>[4x]LSSSPSEILQELGKGSTHPQPGVSPPAAPAAPGPKDGPGETDAFGNSEGKELVASGENKIKQGLLPSLEDLLFYTIAEGQEKIPVHKFITALKSTGLRTSDPRLKECMDMLRLTLQTTSDGVMLDKDLFKKCVQSNIVLLTQAFRRKFVIPDFMSFTSHIDELYESAKKQSGGKVADYIPQLAKFSPD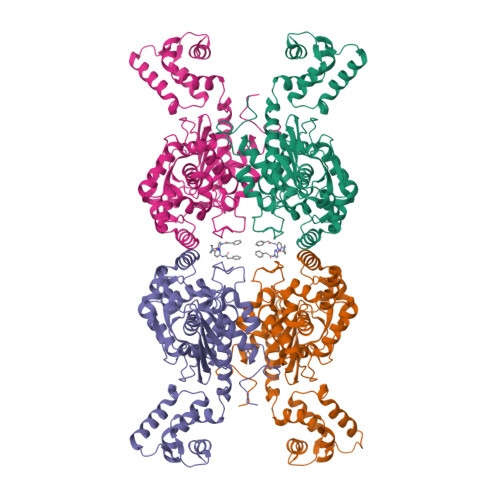LWGVSVCTADGQRHSTGDTKVPFCLQSCVKPLKYAIAVNDLGTEYVHRYVGKEPSGLRFNKLFLNEDDKPHNPMVNAGAIVVTSLIKQGVNNAEKFDYVMQFLNKMAGNEYVGFSNATFQSERESGDRNFAIGYYLKEKKCFPEGTDMVGILDFYFQLCSIEVTCESASVMAATLANGGFCPITGERVLSPEAVRNTLSLMHSCGMYDFSGQFAFHVGLPAKSGVAGGILLVVPNVMGMMCWSPPLDKMGNSVKGIHFCHDLVSLCNFHNYDNLRHFAKKLDPRREGGDQRHSFGPLDYESLQQELALKETVWKKVSPESNEDISTTVVYRMESLGEKS>[2x]QRKLEALIRDPRSPINVESLLDGLNSLVLDLDFPALRKNKNIDNFLNRYEKIVKKIRGLQMKAEDYDVVKVIGRGAFGEVQLVRHKASQKVYAMKLLSKFEMIKRSDSAFFWEERDIMAFANSPWVVQLFYAFQDDRYLYMVMEYMPGGDLVNLMSNYDVPEKWAKFYTAEVVLALDAIHSMGLIHRDVKPDNMLLDKHGHLKLADFGTCMKMDETGMVHC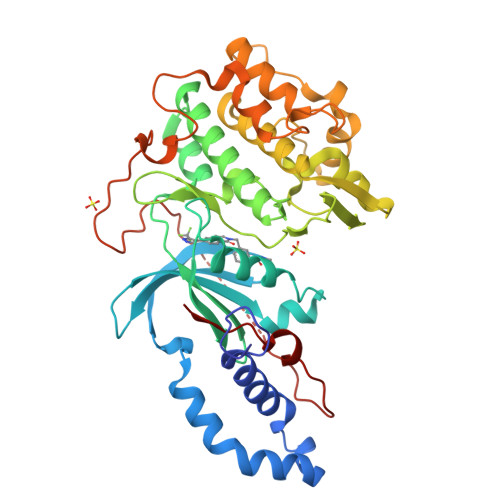DTAVGTPDYISPEVLKSQGGDGFYGRECDWWSVGVFLYEMLVGDTPFYADSLVGTYSKIMDHKNSLCFPEDAEISKHAKNLICAFLTDREVRLGRNGVEEIRQHPFFKNDQWHWDNIRETAAPVVPELSSDIDSSNFDDIEDDKGDVETFPIPKAFVGNQLPFIGFTYYR> EALYVAGYLALYSKD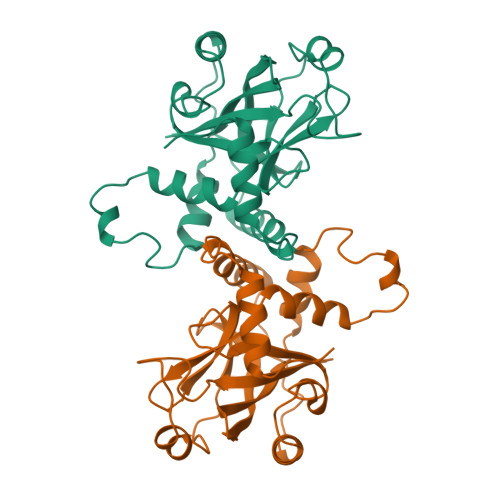EGELNITPEIVRSALPPTSKIPINIDHRKDCVVGEVIAIIEDIRGPFFLGIVRCPQLHAVLFEAAHSNFFGNRDSVLSPLERALYLVTNYLPSVSLSSKRLSPNEIPDGNFFTHVALCVVGRRVGTVVNYDCTPESSIEPFRVLSMESKARLLSLVKDYAGLNKVWKVSEDKLAKVLLSTAVNNMLLRDRWDVVAKRRREAGIMGH> MEYEWKPDEQGLQQILQLLKESQSPDTTIQRTVQQKLEQLNQYPDFN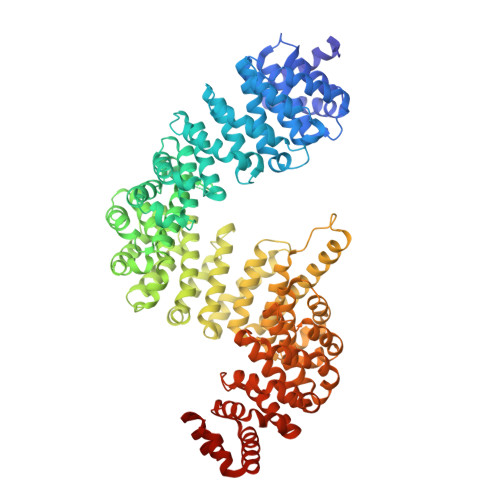NYLIFVLTKLKSEDEPTRSLSGLILKNNVKAHFQNFPNGVTDFIKSECLNNIGDSSPLIRATVGILITTIASKGELQNWPDLLPKLCSLLDSEDYNTCEGAFGALQKICEDSAEILDSDVLDRPLNIMIPKFLQFFKHSSPKIRSHAVACVNQFIISRTQALMLHIDSFIENLFALAGDEEPEVRKNVCRALVMLLEVRMDRLLPHMHNIVEYMLQRTQDQDENVALEACEFWLTLAEQPICKDVLVRHLPKLIPVLVNGMKYSDIDIILLKGDVEEDETIPDSEQDIGGSGGSGDDTISDWNLRKCSAAALDVLANVYRDELLPHILPLLKELLFHHEWVVKESGILVLGAIAEGCMQGMIPYLPELIPHLIQCLSDKKALVRSITCWTLSRYAHWVVSQPPDTYLKPLMTELLKRILDSNKRVQEAACSAFATLEEEACTELVPYLAYILDTLVFAFSKYQHKNLLILYDAIGTLADSVGHHLNKPEYIQMLMPPLIQKWNMLKDEDKDLFPLLECLSSVATALQSGFLPYCEPVYQRCVNLVQKTLAQAMLNNAQPDQYEAPDKDFMIVALDLLSGLAEGLGGNIEQLVARSNILTLMYQCMQDKMPEVRQSSFALLGDLTKACFQHVKPCIADFMPILGTNLNPEFISVCNNATWAIGEISIQMGIEMQPYIPMVLHQLVEIINRPNTPKTLLENTAITIGRLGYVCPQEVAPMLQQFIRPWCTSLRNIRDNEEKDSAFRGICTMISVNPSGVIQDFIFFCDAVASWINPKDDLRDMFCKILHGFKNQVGDENWRRFSDQFPLPLKERLAAFYGV>[4x]MGTISDVKTNVQLLKGRVDNIS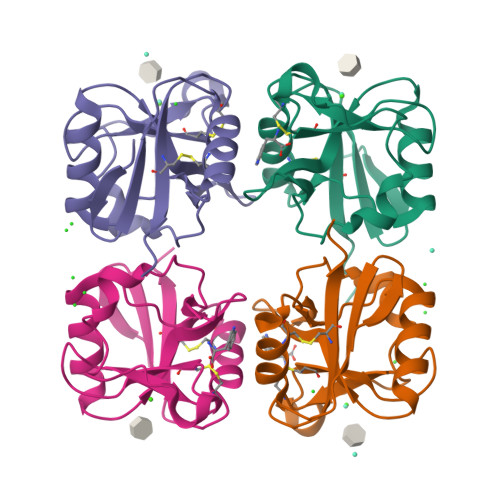TLDSEIKKNSDGMEAAGVQIQMVNESLGYVRSQFLKLKTSVEKANAQIQILTRSWEEVSTLNAQIPELKSDLEKASALNTKIRALQGSLENMSKLLKRQNDILQVVSQGWKYFKGNFYYFSLIPKTWYSAEQFCVSRNSHLTSVTSESEQEFLYKTAGGLIYWIGLTKAGMEGDWSWVDDTPFNKVQSVRFWIPGEPNNAGNNEHCGNIKAPSLQAWNDAPCDKTFLFICKRPYVPSEP> SHMSRKIRDLIESKRFQNVITAIIVLNGAVLGLLTDTTLSASSQNLLERVDQLCLTIFIVEISLK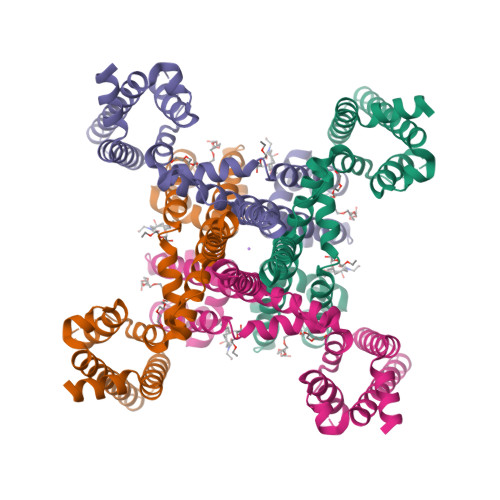IYAYGVRGFFRSGWNLFDFVIVAIALMPAQGSLSVLRTFRIFRVMRLVSVIPTMRRVVQGMLLALPGVGSVAALLTVVFYIAAVMATNLYGATFPEWFGDLSKSLYTLFQVMTLESWSMGIVRPVMNVHPNAWVFFIPFIMLTTLTVLNLFIGIIVDAMAITKEQEEEAKTGHHQEPISQTLLHLGDRLDRIEKQLAQNNELLQRQQPQKK12-(dimethylamino)-3,10-diethyl-N,N,N-trimethyl-3,10-dihydrodibenzo[3,4:7,8]cycloocta[1,2-d:5,6-d']bis([1,2,3]triazole)-5-aminium | C25 H31 N8 | 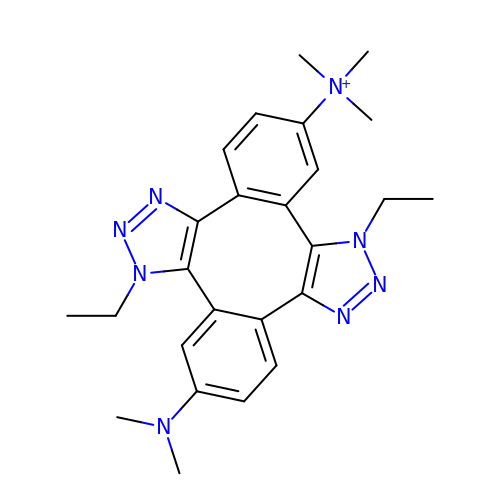QOPAGBBAMAJINO-MOBSCGTJSA-N>[2x]MSSKPKPIEIIGAPFSKGQPRGGVEKGPAALRKAGLVEKLKETEYNVRDHGDLAFVDVPNDSPFQIVKNP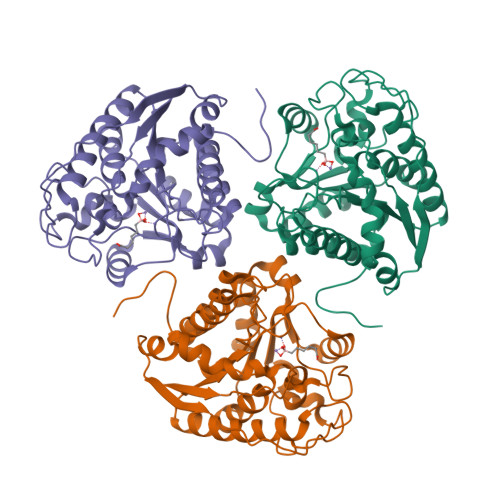RSVGKANEQLAAVVAETQKNGTISVVLGGDHSMAIGSISGHARVHPDLCVIWVDAHTDINTPLTTSSGNLHGQPVAFLLKELKGKFPDVPGFSWVTPCISAKDIVYIGLRDVDPGEHYIIKTLGIKYFSMTEVDKLGIGKVMEETFSYLLGRKKRPIHLSFDVDGLDPVFTPATGTPVVGGLSYREGLYITEEIYKTGLLSGLDIMEVNPTLGKTPEEVTRTVNTAVALTLSCFGTKREGNHKPETDYLKPPK> KQAFLILCLLSAAFAPICVGIVFLGFTPDHHCQSPGVAELSQRCGWSPAEELNYTVPGLGPAGEAFLGQCRRYEVDWNQSALSCVDPLASLATNRSHLPLGPCQDGWVYDTPGSSIVTEFNLVCADSWKLDLFQSCLNAGFLFGSLGVGYFADRFGRKLCLLGTVLVNAVSGVLMAFSPNYMSMLLFRLLQGLVSKGNWMAGYTLITEFVGSGSRRTVAIMYQMAFTVGLVALTGLAYALPHWRWLQLAVSLPTFLFLLYYWCVPESPRWLLSQKRNTEAIKIMDHIAQKNGKLPPADLKMLSLEEDVTEKLSPSFADLFRTPRLRKRTFILMYLWFTDSVLYQGLILHMGATSGNLYLDFLYSALVEIPGAFIALITIDRVGRIYPMAMSNLLAGAACLVMIFISPDLHWLNIIIMCVGRMGITIAIQMICLVNAELYPTFVRNLGVMVCSSLCDIGGIITPFIVFRLREVWQALPLILFAVLGLLAAGVTLLLPETKGVALPETMKDAENLGRKAKPKENTIYLKVQTSEPSGT

Organic Cation Transporter 1 (OCT1), a member of this family primarily localized on the basolateral membrane of hepatocytes, is involved in the uptake of cationic molecules for hepatic metabolism and excretion. Here, we present cryo-EM structures of full-length human OCT1 in the inward-open conformation, both ligand-free and drug-bound, indicating the basis for its broad substrate recognition. The overall architecture of OCT1 in our cryo-EM structures resembles the classical MFS transmembrane arrangement of pseudo-symmetric 6 + 6 transmembrane helical (TM) bundles corresponding to the N-terminal (TMs 1–6) and C-terminal (TMs 7–12) lobes. The structures also show a large extracellular domain (ECD) between TMs 1 and 2 unique to the SLC22 family.

Additionally, anti-arrhythmic drugs such as diltiazem, a calcium channel blocker, exhibiting plasma serum concentrations above the IC50 of OCT1 after administration and could similarly contribute to cardiovascular toxicity. The OCT1-DTZ structure was solved at pH 6.0 as it was necessary to reduce the pH to dissolve diltiazem (due to its lipophilicity and lower pKa of 7.747), but no significant structural changes were observed when OCT1-DTZ was compared to the other structures solved at pH 8.0. In OCT1-DTZ, a pendant ammonium group was close to E386 likely forming an electrostatic interaction. The aromatic groups in OCT1-DTZ were both located near F32, W217, Y361 and I446 which maximized hydrophobic interactions, whereas the additional methoxyphenyl moiety of diltiazem was proximal to W364. Polar interactions between diltiazem and Q241 further stabilize the ligand in the binding site. The hydrophobic pocket of OCT1, with a specific charge coordination through E386, likely favors molecules with a pendant ammonium cation tethered to a large lipophilic or aromatic core. Docking followed by MD simulations of diltiazem (n = 3 × 500 ns replicates) correlated well with the modelling of the cryo-EM map, with an overall RMSD of the ligand of 1.4 ± 0.4 Å calculated across the combined 1500 ns of simulation. On the other hand, the structure of OCT1 in complex with diltiazem (OCT1-DTZ) showed this compound formed electrostatic interactions with E386 through its pendant ammonium cation. In comparison, the smaller localization of a positive charge in the pendant ammonium of OCT1-DTZ generates a stronger interaction with E386 and these compounds are stabilized by additional hydrophobic interactions. Compounds with cationic ammonium pendant groups tethered to an aromatic or hydrophobic core pose significant risks as high-affinity inhibitors of OCT1 as seen in OCT1-DTZ.>[2x]MHHHHHHSSGRENLYFQGLERLDEGLRKEDMAVHVRRDHVFEDSYRELHRKSPEEMKNRLYIVFEGEEGQDAGGLLREWYMIISREMFNP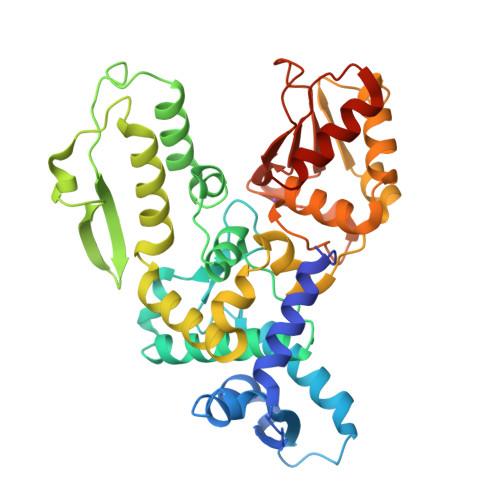MYALFRTSPGDRVTYTINPSSHCNPNHLSYFKFVGRIVAKAVYDNRLLECYFTRSFYKHILGKSVRYTDMESEDYHFYQGLVYLLENDVSTLGYDLTFSTEVQEFGVCEVRDLKPNGANILVTEENKKEYVHLVCQMRMTGAIRKQLAAFLEGFYEIIPKRLISIFTEQELELLISGLPTIDIDDLKSNTEYHKYQSNSIQIQWFWRALRSFDQADRAKFLQFVTGTSKVPLQGFAALEGMNGIQKFQIHRDDRSTDRLPSAHTCFNQLDLPAYESFEKLRHMLLLAIQECSEGFGLA(3R)-3-amino-2,2-difluoro-3-(4-hydroxyphenyl)propanoic acid | C9 H9 F2 N O3 | 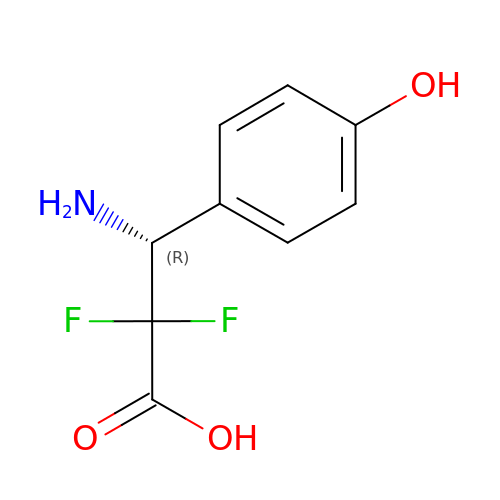GYPNQHABJBHUCN-SSDOTTSWSA-N The LarA family consists of diverse racemases/epimerases that interconvert the diastereomers of a variety of α-hydroxyacids by using a nickel-pincer nucleotide (NPN) cofactor. Accumulating evidence has supported a proton-coupled hydride transfer (PCHT) mechanism for the LarA-catalyzed racemization reaction. According to this hidden redox reaction mechanism, the hydrogen atom on Cα of lactate is transferred as a hydride to the NPN cofactor and then, after a rotation of the acetyl group of the pyruvate intermediate, the hydride returns to Cα to complete racemization. In this work, we report the high-resolution crystal structures of LarA from Isosphaera pallida (LarAIp) in complex with three short-chain aliphatic D-α-hydroxyacids.

We then crystallized LarAIp as purified and solved the structure at 1.74 Å. Two protein molecules are present in one asymmetric unit, but the very small interface (386.2 Å2) does not support a physiological dimer. The well-resolved electron density map at the active site clearly indicated a NPN cofactor tethered to Lys183 through a thioamide bond. Ni is coordinated by two sulfur atoms and C4 of pyridinium ring of the NPN cofactor and the fourth ligand is the Nε of His199, completing a nearly ideal square-planar coordination. On top of the pyridinium ring, a density corresponding to a small molecule was resolved in the structure of LarAIp. The high quality of the electron density allowed us to assign it as D-lactate (a natural substrate of LarAIp) for the best fit of the density. D-lactate is bound at the active site through polar interactions with multiple highly conserved residues (top row). The carboxylic acid group is multi-coordinated with Arg73, Gln295, Lys298, and two catalytic histidine residues His107 and His173, which, together with C2 (or Cα) and the 2-OH group, forms a plane nearly parallel to the pyridinium ring of the NPN cofactor. The rotation of the acetyl group of D-lactate is restricted by the hydrogen bonds between the 2-OH group and residues His107 and Tyr294. Because of these structural constraints, D-lactate is locked in a single conformation with Hα (the hydrogen atom on Cα) pointing toward C4 and Ni of the NPN cofactor with distances of 2.8 Å and 2.9 Å, respectively, allowing a hydride transfer from Cα to the NPN cofactor.

>[2x]RVTLDYGKTGLNVDLPDDRTLPPLTIRPAPPLDDPEAEVVRCLAEPIGSPPLLDLARGKRSACILVCDITRPVPNPVLLRPILRTLHAAGLATQDILILVATGLHRPSTPAEKVEMLSEEIARTYRVEDHYGTRLEEHTYLGTTPNGVPAWIDSRYVQADLKIATGLIEPHLMAGYSGGRKLICPGIAAFETVKLWHGPRFLEHPLADCGFLEGNPVHEENTRIARMAGCDFIVNVTLDGARRITSVVAGDMEQAFLKGVAFVETVVKAAVPAPVDVVVTSSAGHPLDLTFYQAVKGLTGALPIVKPGGTIVIAAALAEGLGSPEFQSLFEEHPTLEGFMEAILKEESFTVDQWQLEELAKVRRKARVKFVSDGVPAAVLSRCHVEPVATVELAVAQALEQYGPEARVAVIPKGPYVLPVVDPTL>[3x]MIVSAIAANALLESVTKFHCGVIYDYSTAEYVSYRPSDFGAYLDALEAEVARGGLIVFHNGHKYDVPALTKLAKLQLNREFHLPRENCIDTLVLSRLIHSNLKDTDMGLLRSGKLPGKRFGSHALEAWGYRLGEMKGEYKDDFKRMLEEQGEEYVDGMEWWNFNEEMMDYNVQDVVVTKALLEKLLSDKHYFPPEIDFTDVGYTTFWSESLEAVDIEHRAAWLLAKQERNGFPFDTKAIEELYVELAARRSE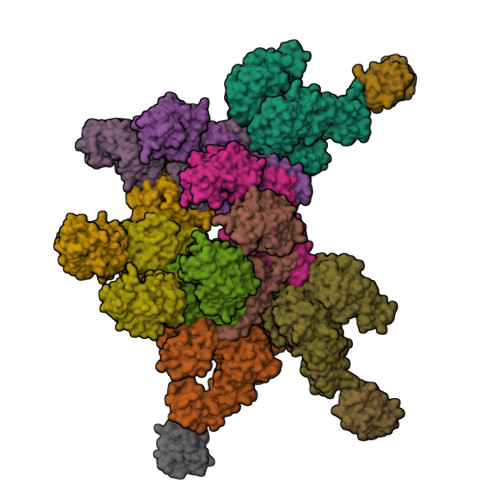LLRKLTETFGSWYQPKGGTEMFCHPRTGKPLPKYPRIKTPKVGGIFKKPKNKAQREGREPCELDTREYVAGAPYTPVEHVVFNPSSRDHIQKKLQEAGWVPTKYTDKGAPVVDDEVLEGVRVDDPEKQAAIDLIKEYLMIQKRIGQSAEGDKAWLRYVAEDGKIHGSVNPNGAVTGRATHAFPNLAQIPGVRSPYGEQCRAAFGAEHHLDGITGKPWVQAGIDASGLELRCLAHFMARFDNGEYAHEILNGDIHTKNQIAAELPTRDNAKTFIYGFLYGAGDEKIGQIVGAGKERGKELKKKFLENTPAIAALRESIQQTLVESSQWVAGEQQVKWKRRWIKGLDGRKVHVRSPHAALNTLLQSAGALICKLWIIKTEEMLVEKGLKHGWDGDFAYMAWVHDEIQVGCRTEEIAQVVIETAQEAMRWVGDHWNFRCLLDTEGKMGPNWAICH;>[7x]MTYNVWNFGESNGRYSALTARGISKETCQKAGYWIAKVDGVMYQVADYRDQNGNIVSQKVRDKDKNFKTTGSHKSDALFGKHLWNGGKKIVVTEGEIDMLTVMELQDCKYPVVSLGHGASAAKKTCAANYEYFDQFEQIILMFDMDEAGRKAVEEAAQVLPAGKVRVAVLPCKDANECHLNGHDREIMEQVWNAGPWIPDGVVSALSLRERIREHLSSEESVGLLFSGCTGINDKTLGARGGEVIMVTSGSGMGKSTFVRQQALQWGTAMGKKVGLAMLEESVEETAEDLIGLHNRVRLRQSDSLKREIIENGKFDQWFDELFGNDTFHLYDSFAEAETDRLLAKLAYMRSGLGCDVIILDHISIVVSASGESDERKMIDNLMTKLKGFAKSTGVVLVVICHLKNPDKGKAHEEGRPVSITDLRGSGALRQLSDTIIALERNQQGDMPNLVLVRILKCRFTGDTGIAGYMEYNKETGWLEPSSYSG;>KIIHLTDDSFDTDVLKADGAILVDFWAEWCGPCKMIAPILDEIADEYQGKLTVAKLNIDQNPGTAPKYGIRGIPTLLLFKNGEVAATKVGALSKGQLKEFLDANL[3x]>MNMDWALFLTFLAACGAPATTGALLKPDEWYDNLNKPWWNPPRWVFPLAWTSLYFLMSLAAMRVAQLEGSGQALAFYAAQLAFNTLWTPVFFGMKRMATALAVVMVMWLFVAATMWAFFQLD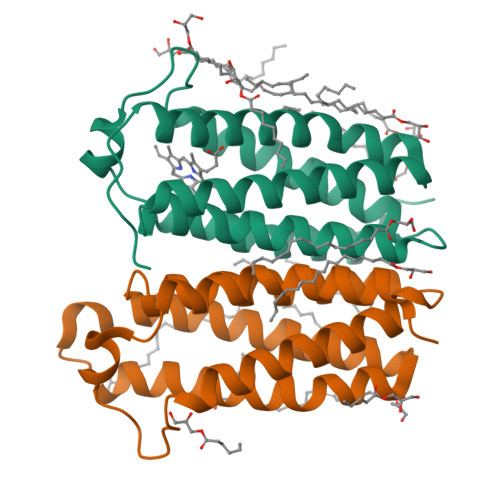TWAGVLFVPYLIWATATTGLNFEAMRLNWNRPEAR[3x]>MTAPRSWAPTTRARGDTEALCSPEDGWVKVHPTPGTMLFREILHGQLG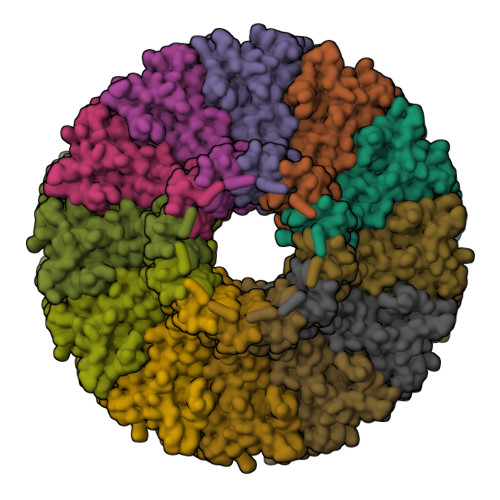YTEGQGVYNVVRSSEATTRQLQAAIFHALLNATTYRDLEADWLGHVAARGLQPQRLVRRYRNAREADIAGVAERVFDTWRNTLRTTLLDFAHGLVACFAPGGPSGPSSFPKYIDWLTCLGLVPILRKRQEGGVTQGLRAFLKQHPLTRQLATVAEAAERAGPGFFELALAFDSTRVADYDRVYIYYNHRRGDWLVRDPISGQRGECLVLWPPLWTGDRLVFDSPVQRLFPEIVACHSLREHAHVCRLRNTASVKVLLGRKSDSERGVAGAARVVNKVLGEDDETKAGSAASRLVRLIINMKGMRHVGDINDTVRAYLDEAGGHLIDAPAVDGTLPGFGKGGNSRGSAGQDQGGRAPQLRQAFRTAVVNNINGVLEGYINNLFGTIERLRETNAGLATQLQERDRELRRATAGALERQQRAADLAAESVTGGCGSRPAGADLLRADYDIIDVSKSMDDDTYVANSFQHPYIPSYAQDLERLSRLWEHELVRCFKILCHRNNQGQETSISYSSGAIAAFVAPYFESVLRAPRVGAPITGSDVILGEEELWDAVFKKTRLQTYLTDIAALFVADVQHAALPPPPSPVGADFRPGASPRGRSRSRSPGRTAPGAPDQGGGIGHRDGRRDGRR[12x]> KNTVSIFALGPTITDDDEKMTLALLFLSHSLDNEKQHAQRAGFLVSLLSMAYANPELYLTTNGSNADVKYVIYMIEKDLKRQKYGGFVVKTREMIYEKTTEWIFGSDLDYDQETMLQNGRNNSTIEDLVHTFGYPSCLGALIIQIWIVLVKAITSISGLRKGFFTRLEAFRQDGTVQAGLVLSGDTVDQIGSIMRSQQSLVTLMVETLITMNTSRNDLTTIEKNIQIVGNYIRDAGLASFFNTI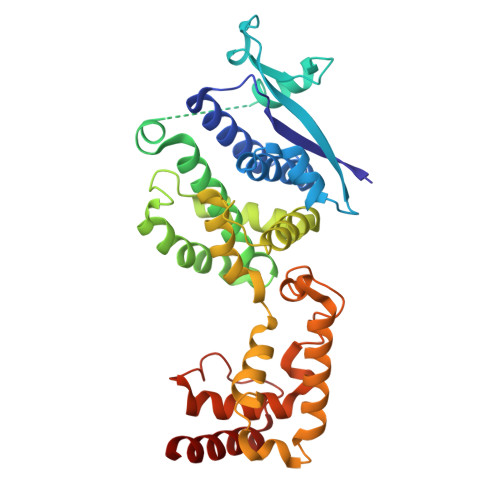RYGIETRMAALTLSTLRPDINRLKALMELYLSKGPRAPFICILRDPIHGEFAPGNYPAIWSYAMGVAVVQNRAMQQYVTGRSYLDIDMFQLGQAVARDAEAQ> GSNGVSEAELLTKTLPDILTFNLDIVIIGINPGLM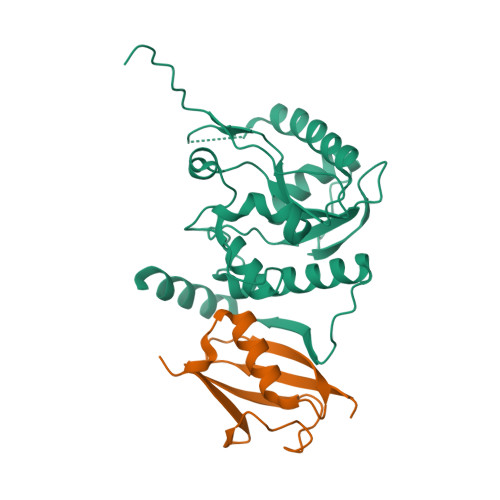AAYKGHHYPGPGNHFWKCLFMSGLSEVQLNHMDDHTLPGKYGIGFTNMVERTTPGSKDLSSKEFREGGRILVQKLQKYQPRIAVFNGKCIYEIFSKEVFGVKVKNLEFGLQPHKIPDTETLCYVMPSSSARCAQFPRAQDKVHYYIKLKDLRDQLKGIERNMDVQEVQYTFDLQLAQEDAKKMAVKEEKYDPGYE;> MADEKPKEGVKTENNDHINLKVAGQDGSVVQFKIKRHTPLSKLMKAYCERQGLSMRQIRFRFDGQPINETDTPAQLEMEDEDTIDVFQQQTGG>SMADGNEDLRADDLPGPAFESYESMELACPAERSGHVAVSDGRHMFVWGGYKSNQVRGLYDFYLPREELWIYNMETGRWKKINTEGDVPPSMSGSCAVCVDRVLYLFGGHHSRGNTNKFYMLDSRSTDRVLQ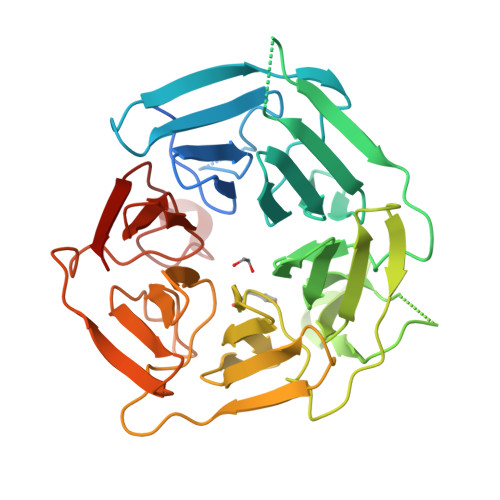WERIDCQGIPPSSKDKLGVWVYKNKLIFFGGYGYLPEDKVLGTFEFDETSFWNSSHPRGWNDHVHILDTETFTWSQPITTGKAPSPRAAHACATVGNRGFVFGGRYRDARMNDLHYLNLDTWEWNELIPQGICPVGRSWHSLTPVSSDHLFLFGGFTTDKQPLSDAWTYCISKNEWIQFNHPYTEKPRLWHTACASDEGEVIVFGGCANNLLVHHRAAHSNEILIFSVQPK[2x]>APITAYSQQTRGLLGCIITSLTGRDKNQVEGEVQVVSTATQSFLATCVNGVCWTVYHGAGSKTLAGPKGPITQMYTNVDQDLVGWQAPPGARSLTPCTCGSSDLYLVTRHADVIPVRRRGDSRGSLLSPRPVSYLKGSSGGPL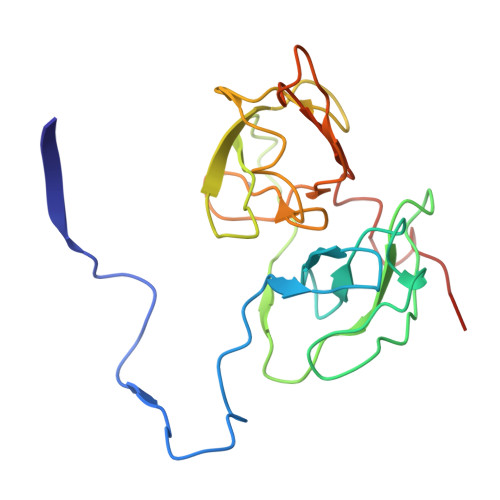LCPSGHAVGIFRAAVCTRGVAKAVDFVPVESMETTMRSPVFTDNSS[3x]>[4x]SQLLNYIDGNFVTSASSFANINPVNGKLISDVFEADAKQVNEAVVAAQNALKGPWGKLSVQDRAALIHKIADGIQARFEEFVAAEVADTGRPVHQARTL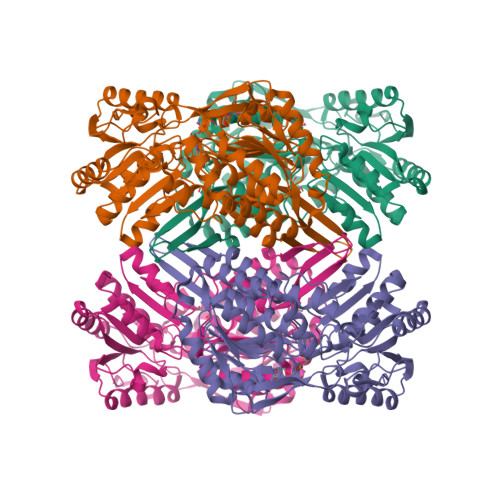DIPRAIANFRTFADLAKTSHTDLFEMSTSDGSGALNYTVRKPLGVIGVISPWNLPLLLFTWKVAPALACGNTVVAKPSEESPSSATLLAEVMHDAGVPPGVFNLIHGFGKDSAGEFLTQHPGISALTFTGESKTGSTIMKAVADGVKEVSFALGGKNAAVVFADADLDAAIEGVLRSSFTNSGQVCLCSERVYVHRSIFDEFVSGLKVEAERLVVGYPDQDGVNMGPLISHGHRDKVLSYYRLAVDEGATVVTGGGVPKFNDERDQGAYVQPTIWTGLSDKARCVTEEIFGPVCHISPFDDEDEVINRVNDSNYGLACAIWTTNLSRAHRVSRQIHVGLVWVNTWYLRDLRTPFGGVKLSGLGREGGRFSMDFYSDIANICIKI>[2x]MRVFPVTLGPLQENAYLVETGEGPVLIDPGDEPEK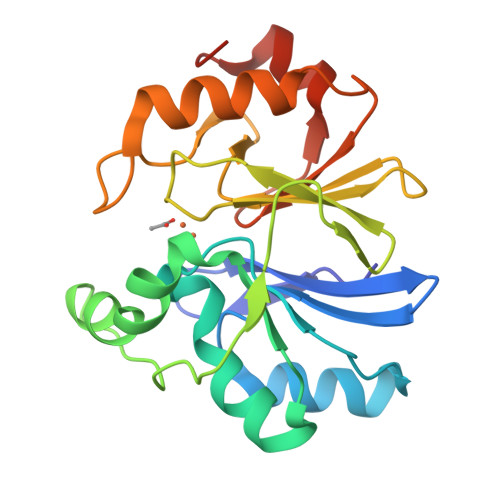LLALFQTTGLIPLAILLTHAHFDHVGAVAPLVEALDLPVYLHPLDLPLYEGADLAARAWGLAIPKPPLPVRPLEEGMRLFGFQVLHLPGHSPGHVAFYDPEGAQVFSGDLLFRGSVGRYDLPGADPKALFASLKRLLSLPPETRVHPGHGPGTTLGLEARTNPFLTGLEWEA> STNDNIKDL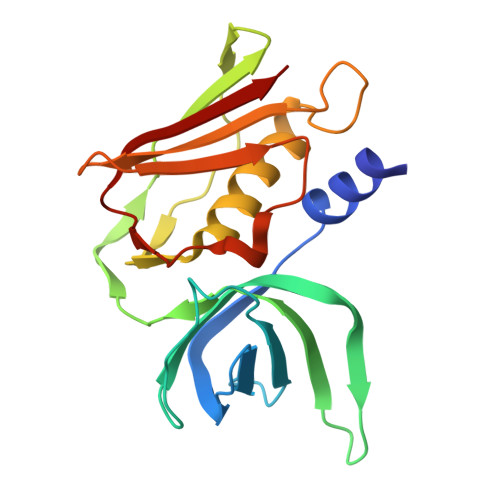LDWYSSGSDTFTNSEVLDNSLGSMRIKNTDGSISLIIFPSPYYSPAFTKGEKVDLNTKRTKKSQHTSEGTYIHFQISGVTNTEKLPTPIELPLKVKVHGKDSPLKYWPKFDKKQLAISTLDFEIRHQLTQIHGLYRSSDKTGGYWKITMNDGSTYQSDLSKKFEYNTEKPPINIDEIKTIEAEIN>[10x]MKPVSLSYRCPCRFFESHVARANVKHLKILNTPNCALQIVARLKNNNRQVCIDPK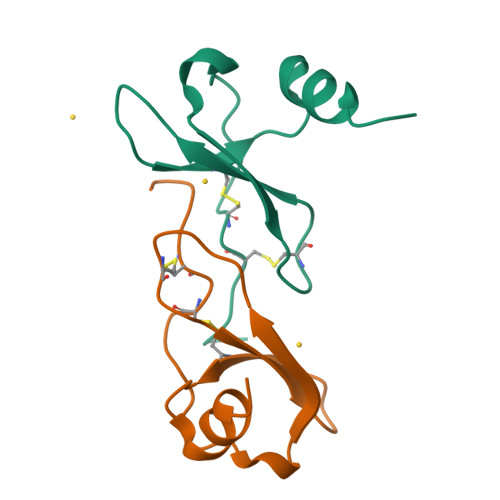LKWIQEYLEKALN>GSNEIKRGAVDLIKTGVNEKAMAGAVFSLFKKDGTEVKKELATDANGHIRVQGLEYGEYYFQETKAPKGYVIDPTKREFFVKNSGTINEDGTITSGTVVKMEVKNNEEPTIDKKINGKLEALPINPLTNYNYDIKTLIPEDIKEYKKYVVTATLDNRLVIQGKPIVKIDGAEVNANVVEVAIEGQKVTATVKDFTKMDGKKEFHLQIKSQVKEGVPSGSEILNTAKIHFTNKNDVIGEKESKPVVVIPTTGIIELTKIDSANKNKMKGAEFVLKDNNGKIVVVAGKEVTGVSDENGVIKWSNIPYGDYQIFETK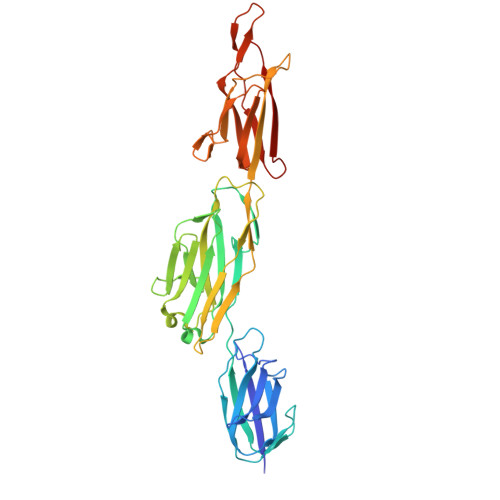APTYTKEDGTKTSYQLLKDPIDVKISENNQTVKLTIENNKS[2x]>MKEWQENKSWNAHFTEHKSQGVVVLWNENKQQGFTNNLKRANQAFLPASTFKIPNSLIALDLGVVKDEHQVFKWDGQTRDIATWNRDHNLITAMKYSVVPVYQEFARQIGEARMSKMLHAFDYGNEDISGNVDSFWLDGGIRISATEQISFLRKLYHNKLHVSERSQRIVKQAMLTEANGDYIIRAKTGYSPKI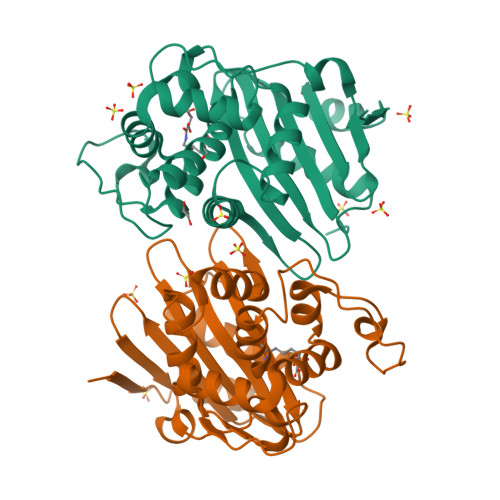GWWVGWVELDDNVWFFAMNMDMPTSDGLGLRQAITKEVLKQEKIIPLEHHHHHHHH[2x]> MEVYRRITERVRGALWAHHGRLMSERQFHRILAYVYNNKYEHQIRFDRMEVVGRAWEGRVEVVTTPAGYLKRVRVNPCLEELSSYRQQQLILAAYADACAQGRRLMEKAEINIYKQFLKDLKPIVMGIRDNPEFYTVPEDSVETVGGTLHMGQGPTPTTYRTIPAAKAHIPVDEIRARQEWEKKWLNSPQGQSWALTLRGKRYFALHGPQYRPRGAPGAKKVTMPLDLPAPYTSMDERRLLKKNWMAYLDNKHVAE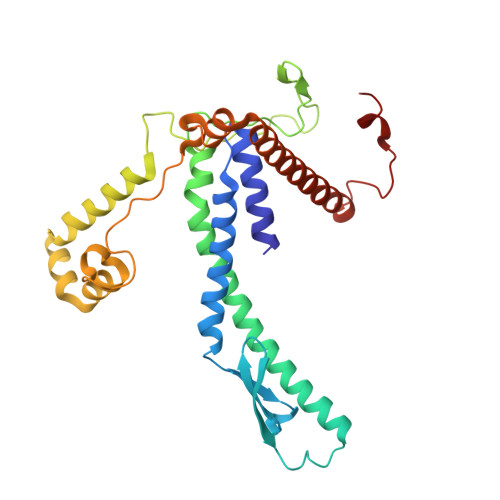VMWTRAKIADREKLQRRLQETGQAWHRPINKEAVSRW> PGSAMAKKINDDIKYQLMKEVRRFGQNYER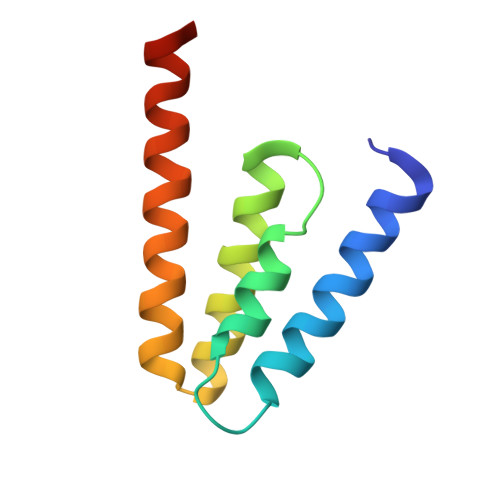IFILLEEVQGSMKVKRQFVEFTIKEAARFKKVVLIQQLEKALKEIDSHCHLRKVKHMRKR>[2x]MRGLLVLSVLLGAVFGKEDFVGHQVLRISVADEAQVQKVKELEDLEHLQLDFWRGPAHPGSPIDVRVPFPSIQAVKIFLESHGISYETMIEDVQSLLDEEQEQMFAFRSRARSTDTFNYATYHTLEEIYDFLDLLVAENPHLVSKIQIGNTYEGRPIYVLKFSTGGSKRPAIWIDTGIHSREWVTQASGVWFAKKITQDYGQDAAFTAILDTLDIFLEI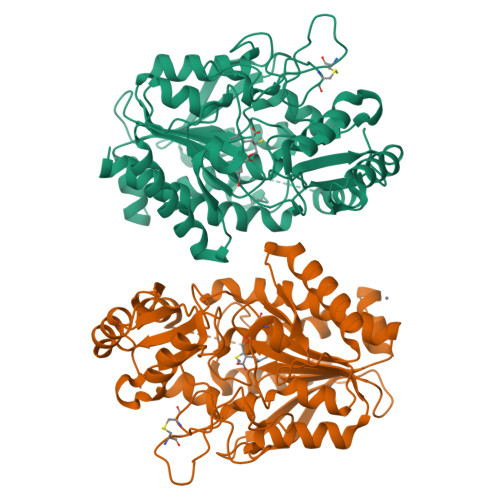VTNPDGFAFTHSTNRMWRKTRSHTAGSLCIGVDPNRNWDAGFGLSGASSNPCSETYHGKFANSEVEVKSIVDFVKDHGNIKAFISIHSYSQLLMYPYGYKTEPVPDQDELDQLSKAAVTALASLYGTKFNYGSIIKAIYQASGSTIDWTYSQGIKYSFTFELRDTGRYGFLLPASQIIPTAKETWLALLTIMEHTLNHPY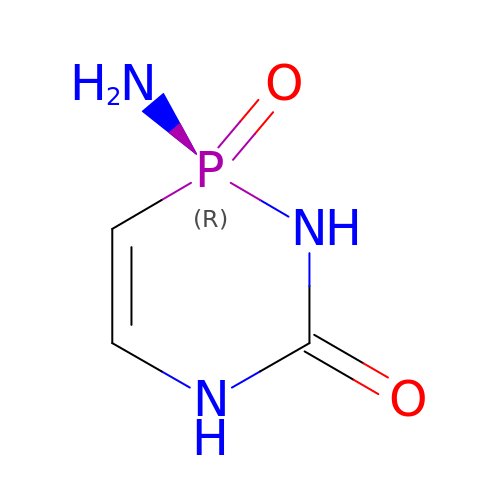(2R)-2-amino-2,5-dihydro-1,5,2-diazaphosphinin-6(1H)-one 2-oxide | C3 H6 N3 O2 P | GGLLBAYBJJLFCT-SECBINFHSA-N>AQDMVSPPPPIADEPLTVNTGIYLIECYSLDDKAETFKVNAFLSLSWKDRRLAFDPVRSGVRVKTYEPEAIWIPEIRFVNVENARDADVVDISVSPDGTVQYLERFSARVLSPLDFRRYPFDSQTLHIYLIVRSVDTRNIVLAVDLEKVGKNDDVFLTGWDIESFTAVVKPANFALEDRLESKLDYQLRISRQYFSYIPNIILPMLFILFISWTAFWSTSYEANVTLVVSTLIAHIAANILVETNLPKTPYMTYTGAIIFMIYLFYFVAVIEVTVQHY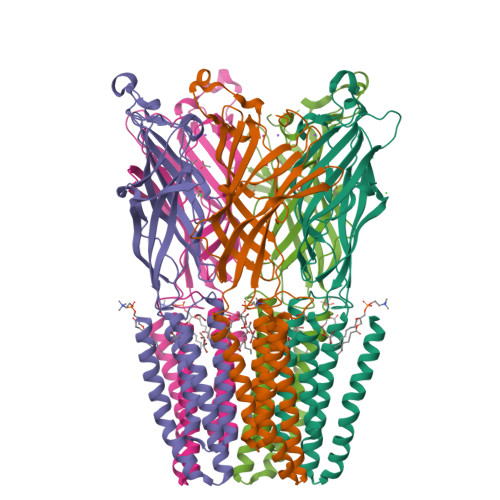LKVESQPARAASITRASRIAFPVVFLLANIILAFLFFGF[5x]5,8-dimethoxy-1,4-dimethylquinolin-2(1H)-one | C13 H15 N O3 | 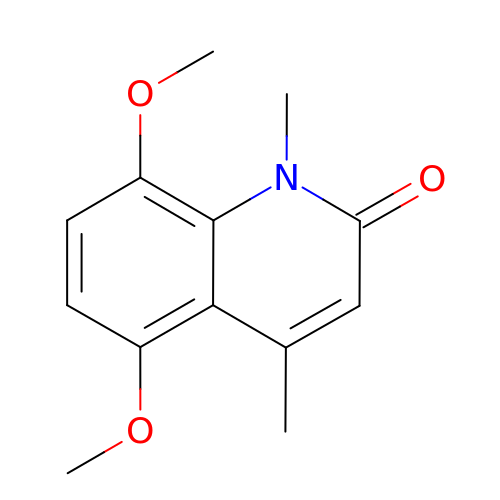FTGZPMFPUDKJBX-UHFFFAOYSA-N>MKITSSNFATIATSENFAKLSVLPKNHREPIKGLFKSAVEQFSSARDFFKNENYSKELAEKFNKEAVNEAVEKLQKAIDLAEKQGIQFLEHH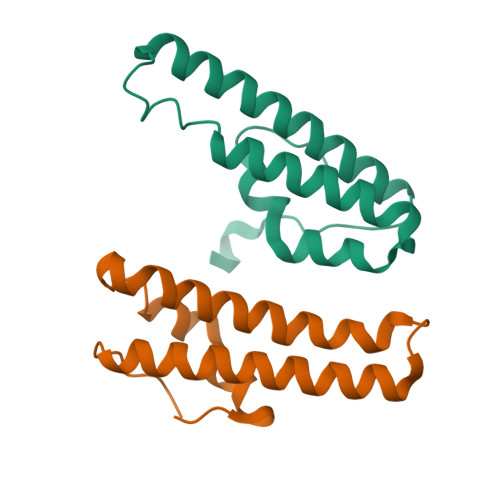HHHH[2x]> ETGATTGPKVLCYYDGQMSLREGLGKITVTDIELALPFCTHLLYGFAGVNPETYRLKALDESLELDSGKGQYRLATTLKRRYPNLKVLLSVGGYKDLTEEKPFEKYLTLLESAGSRTAFVNSVYSTLKTYDFDGLDLAWQFPQTKPKRIRGWTGKVWHGFKKLFTGDSVLDPEADEHREEFTALVRDLKNALVADNFILGLTVLPHVNESIFMDVPLLKDNLDYVNLASFDQQTPERNPKEGDYTAPIYEPSERVEGNNVDAEASYWLKQGTPAGKIVIGIPTYGRGWKLVEKSGITGVPPIPADGPSIPGPHSGINGFYSWAEVCAKLPNPGNANLQGADQPLRKIGDPTRRFGAYAFRIPDENEEHGIWLSYEDPDTAGNKAAYVKAKGLGGISIFDLGNDDVRGACAGDKFPILRAAKYRLKHHHHHH

Recently, two additional Aedes aegypti proteins, A. aegypti bacteria-responsive 1 (AgBR1) and neutrophil stimulating factor 1 (NeSt1), have been described as inductors of neutrophil recruitment at the bite site, enhancing the dissemination of the virus during the early infection of ZIKV. No structural information exists on AgBR1, but based on its primary amino acid sequence, AgBR1 belongs to the glycoside hydrolase 18 (GH18) family of chitinases. The crystal structure of AgBR1 shows a triose-phosphate isomerase (TIM) barrel with eight α-helices surrounding eight β-strands, a fold conserved across the GH18 family. We propose that in Aedes aegypti, AgBR1 functions as a signaling protein when injected into human skin, based on its described structure and physicochemical properties.

The crystal structure of HCM AgBR1 was determined to 1.2 Å resolution, demonstrating AgBR1 to possess a glycoside hydrolase family 18 (GH18) chitinase fold. The core domain is a classical TIM barrel composed of eight parallel β-barrels (β1-β8) surrounded by eight α-helices (α1-α8) antiparallel to the barrel. The insertion domain formed by an additional α+β-fold between the β7 and α7 (residues Y302-Y391 compared to Imaginal Disc Growth Factor-2, IDGF-2) defines AgBR1 to belong to the subfamily A. The consensus motif of GH18 chitinases active site is DXXDXDXE, located in the β4 strand. The key conserved glutamic acid residue, acting as proton donor during hydrolysis of the glycoside bond, is substituted by Q (E157Q). In AgBR1, the D residue preceding Q157 in the motif, which stabilizes the catalytic amino acid and is part of the substrate-binding cleft, is substituted by A155 (right inset). These mutations lead to the loss of activity that catalyzes the hydrolysis of chitin. The achieved high resolution also resolves the only N-glycosylation site at the N207 residue, which shows two ordered N-acetylglucosamine (NAG) carbohydrates linked by a β(1-4) linkage, with the distal one being more flexible (left inset). Only one region of the AgBR1 molecule in the crystal structure (residues R165-V186), which corresponds to a loop between β4 and α4, displays weak electron density supporting a high degree of flexibility. Furthermore, we identified a K190E mutation, resulting from a missense mutation at the nucleotide level of the Ho Chi Minh strain of mosquitoes compared to the Liverpool strain (LVP). In fact, the superimposition of AgBR1 with the crystal structure of the CHI3L2-chitooligosaccharide complex indicates that its putative ligand-binding site is smaller and exhibits clashes with the ligand primarily caused by loops 2 and 4.>[2x]MFQTFEGD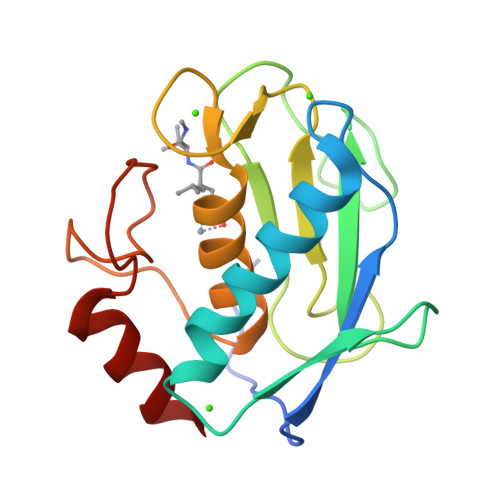LKWHHHNITYWIQNYSEDLPRAVIDDAFARAFALWSAVTPLTFTRVYSRDADIVIQFGVAEHGDGYPFDGKDGLLAHAFPPGPGIQGDAHFDDDELWSLGKGQGYSLFLVAAHEFGHALGLDHSSVPEALMYPMYRFTEGPPLHKDDVNGIRHLY>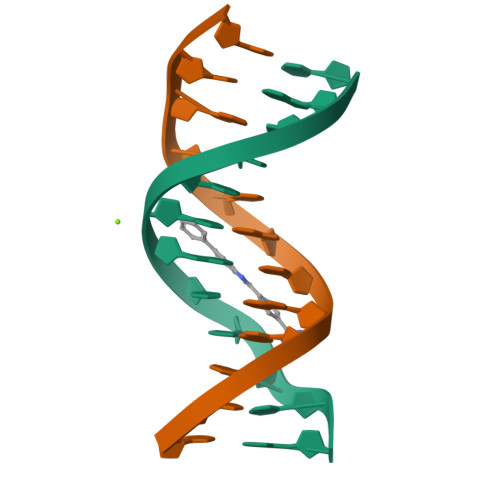CGCGATATCGCG[2x]> GSMRHILERPDPTDVFQNKAAVCWAKALVPVLKTAGIDMTTEQWNTVDYFETDKAHSAEIVLNQLCVRFFGLDLDSGLFSAPTVPLSIRNNHWDNSPSPNMYGLNKEVVRQLSRRYPQLPRAVATGRVYDMNTGTLRNYDPRINLVPVNRRLPHALVLHHNEHPQSDFSSFVSKLKGRTVLVVGEKLSVPGKMVDWLSDRPEATFRARLDLGIPGDVPKYDIIFVNVRTPYKYHHYQQCEDHAIKLSMLTKKACLH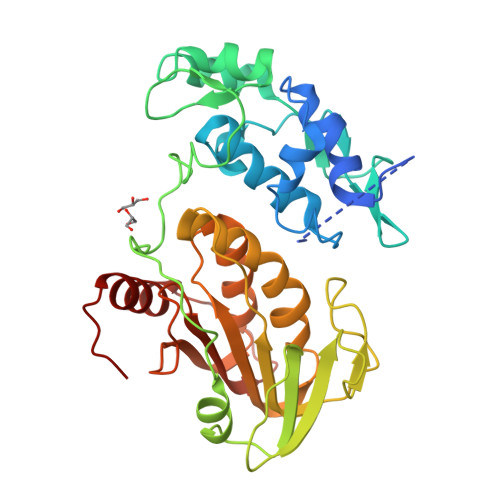LNPGGTCVSIGYGYADRASESIIGAIARQFKFSRVCKPKSSLEETEVLFVFIGYDRKARTHNPYKLSSTLTNIYTGSRLHEA6-azanyl-2-cyclohexyl-4-fluoranyl-1~{H}-pyrrolo[3,4-c]pyridin-3-one 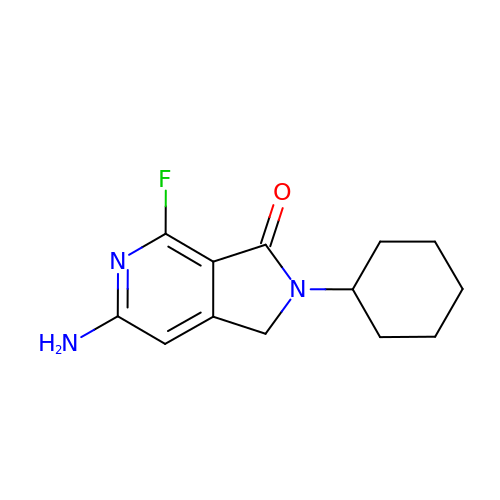| C13 H16 F N3 O | SMGICYCLIWZBPC-UHFFFAOYSA-N> MGSDKIHHHHHHMRIHVLCDDSSQNGFESEHGFSVLVDSVLFDTGKSDVFLKNARKL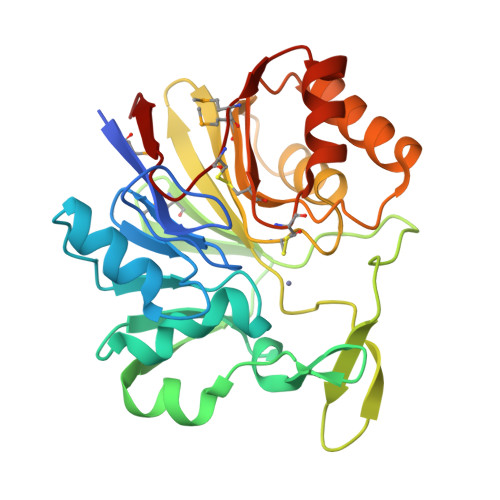GIDLPKDVLISHGHYDHAGGLLYLSGKRVWLRKEALDQKYSGERYAGADWNEVLYYNTGKFVIERITEIGKNMFLLGPANLRGKVPTGDFFVERNGERRKDLFEDEQTLVVRTKEGLVVITGCSHRGIDNILLDIAETFNERIKMVVGGFHLLKSSDDEIEKIVKAFNELGVETVVPCHCTGERAVDIFKREFLGKIMDCYAGLKLEVSD> GSDQEAKPSTEDLGDKKEGEYIKLKVIGQDSSEIHFKVKMTTHLKKLKESYAQRQ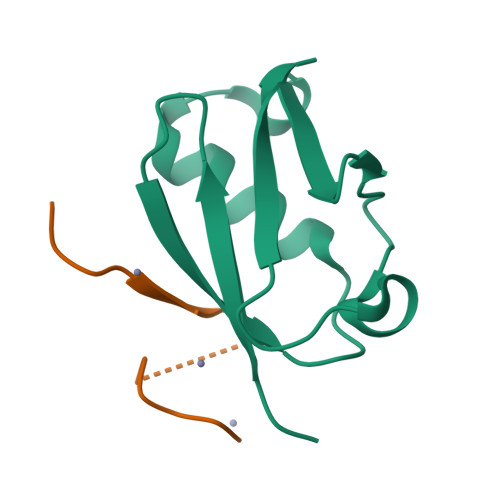GVPMNSLRFLFEGQRIADNHTPKELGMEEEDVIEVYQEQTGG;> GSGAGEAEERVVVISSSEDSDAENSSSRY> KTSAAAQLDELMAHLTE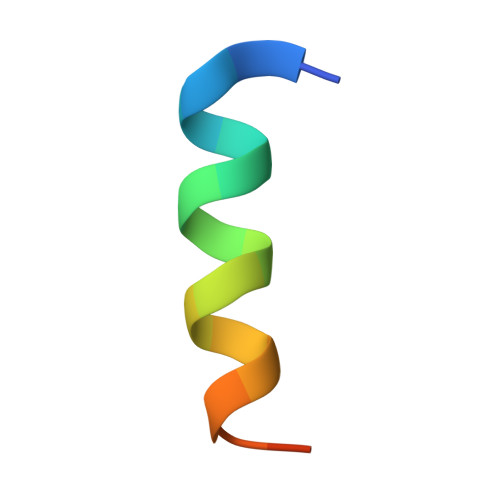MQ>MAPMLSGLLARLVKLLLGRHGSALHWRAAGAAT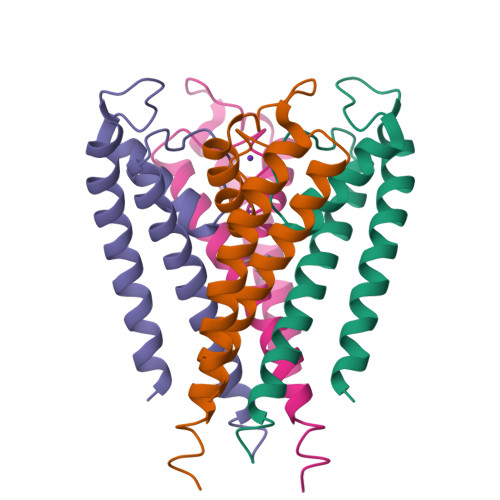VLLVIVLLAGSYLAVLAERGAPGAQLITYPRALWWSVETATTVGYGDLYPVTLWGRCVAVVVMVAGITSFGLVTAALATWFVGREQERRGHF[4x]We later discovered that H. pylori encodes an atypical species‐specific bifunctional dehydrogenase/isomerase enzyme FabX, which introduces a cis‐double bond to the saturated acyl substrate of ACP via a backtracking mechanism that expectedly reverses the conventional fatty acid elongation direction. FabX utilizes a nitronate monooxygenase (NMO) flavoprotein family conserved flavin mononucleotide (FMN) cofactor and an active residue His182 inside the catalytic tunnel to extract electrons/protons from the acyl substrate for dehydrogenation and cis‐double bond formation, storing the captured electrons in FMN and [4Fe‐4S] cluster cofactors, respectively. Subsequently, FabX transfers the stored electrons back to the oxygen molecule located in the oxyanion hole between FMN and His182, generating superoxide (ROS), which is further excreted by H. pylori as a major source of peroxide, likely enabling its pathogenic function of gastric mucosa corrosion. Here, it is demonstrated that FabX is essential for H. pylori growth and gastric colonization by retaining UFA synthesis and producing ROS, respectively, and is a species‐specific anti‐H. pylori drug target.

Subsequently, we examined the enzymatic activities of these compounds and found that 8p (annotated as FBX‐1991, hereinafter) exhibited an outstanding inhibitory activity against FabX with an IC 50 value of 0.158 ± 0.030 × 10−6 m in vitro, and increased the stability of FabX by ≈18.2 °C (ΔTm) at a concentration of 50 × 10−6 m. In contrast, it does not inhibit the enzymatic activities of the structurally conserved homolog FabK, the functionally conserved homolog FabI and the conventional UFA synthase FabA at compound concentrations of up to 10 × 10−6 m compound concentration, indicating a high selectivity of FBX‐1991 against FabX. To elucidate the inhibition mechanism of FBX‐1991 against FabX, we determined the X‐ray crystal structure of FabX in complex with FBX‐1991 in space group P21 at a resolution of 2.00 Å resolution. Subsequent structural analysis indicated that FBX‐1991 binds in the region between the FMN cofactor and the catalytic tunnel of FabX surrounded by α10, α14‐α16, β3‐β6, β9, and β10, and inserts its 2,4‐dichlorophenyl group into the catalytic tunnel, pointing towards the bottom of the tunnel near the [4Fe‐4S] cluster. In the structure of FabX–FBX‐1991 complex, FBX‐1991 is stabilized in the catalytic tunnel predominantly through hydrophobic interactions. The methyl benzoate of FBX‐1991 (A moiety) interacts with the isoalloxazine ring of FMN via π–π interactions. Meanwhile, the carboxyl group of the methyl benzoate group forms an H‐bond with the sidechain of Arg280 located at the N‐terminus of FabX β10 strand, which further stabilizes the methyl benzoate in the correct position.

> GSMVSTLKPLKIGKHTIKFPIFQGGMGVGISWDELAGNVAKEGALGVISAVGTGYYKNMRFVERIVAKKPFEALNFYSKKALNEIFANARKICGNNPLGANILYAINDYGRVLRDSCEAGANIIITGAGLPTNMPEFAKDFSDVALIPIISSAKALKILCKRWSDRYKRIPDAFIVEGPLSGGHQGFKYEDCFKEEFRLENLVPKVVEASKEWGNIPIIAAGGIWDRKDIDTMLSLGASGVQMATRFLGTKECDAKVYADLLPTLKKEDILLIKSPVGYPARAINTGVIKRIEEGNAPKIACVSNCVAPCNRGEEAKKVGYCIADGLGRSYLGNREEGLYFTGANGYRVDKIISVHELIKELTEG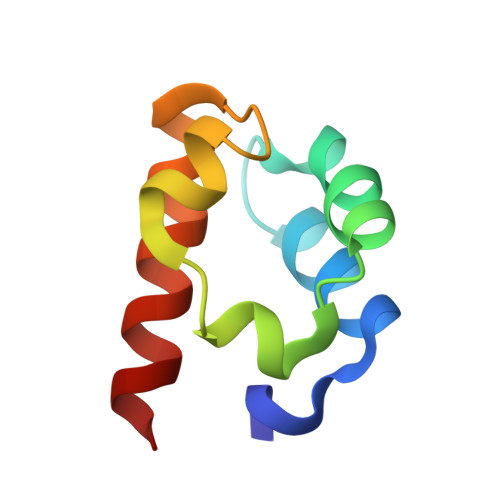> SVSKWSTDEVSEFIQSLPGCEEHGKVFKDEQIDGEAFLLMTQTDIVKIMSIKLGPALKIFNSILMFKAAE GLUTAMINE HYDROXAMATE | C5 H10 N2 O4 | 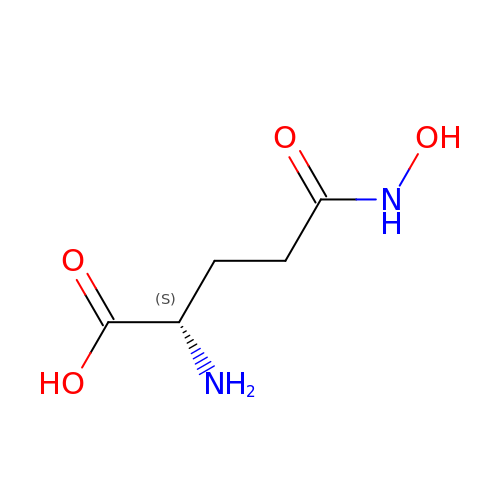YVGZXTQJQNXIAU-VKHMYHEASA-N> MTVRKNQATLTADEKRRFVAAVLELKRSGRYDEFVRTHNEFIMSDTDSGERTGHRSPSFLPWHRRFLLDFEQALQSVDSSVTLPYWDWSADRTVRASLWAPDFLGGTGRSTDGRVMDGPFAASTGNWPINVRVDSRTYLRRSLGGSVAELPTRAEVESVLAISAYDLPPYNSASEGFRNHLEGWRGVNLHNRVHVWVGGQMATGVSPNDPVFWLHHAY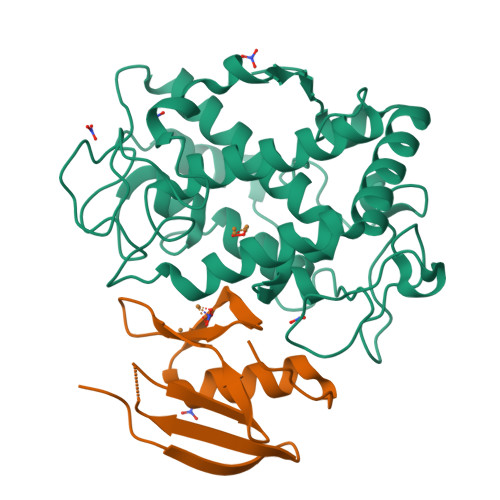VDKLWAEWQRRHPDSAYVPTGGTPDVVDLNETMKPWNTVRPADLLDHTAYYTFDALEHHHHHH;> MPEITRRRALTAAAAVAATASAAVTLAAPAASAAGHHEPAAPESFDEVYKGRRIQGRPAGGGAHHHEHGGGYEVFVDGVQLHVMRNADGSWISVVSHFDPVPTPRAAARAAVDELQGAPLLPFPANLEHHHHHH5-methyl-3-(1-methyl-1H-imidazol-5-yl)-7-(2-methylpropyl)-2-(naphthalen-1-ylmethyl)-2H-pyrazolo[3,4-d]pyrimidine-4,6(5H,7H)-dione 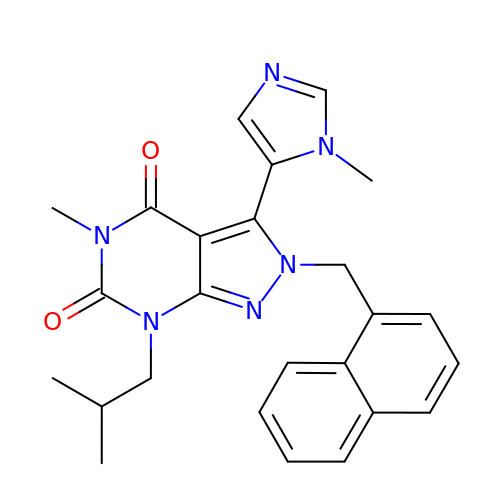| C25 H26 N6 O2 | QJBUEINIMXZUED-UHFFFAOYSA-N>MLGTGPAAATTAATTSSNVSVLQQFASGLKSRNEETRAKAAKELQHYVTMELREMSQEESTRFYDQLNHHIFELVSSSDANERKGGILAIASLIGVEGGNATRIGRFANYLRNLLPSNDPVVMEMASKAIGRLAMAGDTFTAEYVEFEVKRALEWLGADRNEGRRHAAVLVLRELAISVPTFFFQQVQPFFDNIFVAVWDPKQAIREGAVAALRACLILTTQREPKEMQKPQWYRHTFEEAEKGFDETLAKEKGMNRDDRIHGALLILNELVRISSMEGERLREEMEEITQQQLVHDKYCKDLMGFGTKPRHITPFTSFQAVQPQQSNALVGLLGYSSHQGLMGFGTSPSPAKSTLVESRCCRDLMEEKFDQVCQWVLKCRNSKNSLIQMTILNLLPRLAAFRPSAFTDTQYLQDTMNHVLSCVKKEKERTAAFQALGLLSVAVRSEFKVYLPRVLDIIRAALPPKDFAHKRQKAMQVDATVFTCISMLARAMGPGIQQDIKELLEPMLAVGLSPALTAVLYDLSRQIPQLKKDIQDGLLKMLSLVLMHKPLRHPGMPKGLAHQLASPGLTTLPEASDVGSITLALRTLGSFEFEGHSLTQFVRHCADHFLNSEHKEIRMEAARTCSRLLTPSIHLISGHAHVVSQTAVQVVADVLSKLLVVGITDPDPDIRYCVLASLDERFDAHLAQAENLQALFVALNDQVFEIRELAICTVGRLSSMNPAFVMPFLRKMLIQILTELEHSGIGRIKEQSARMLGHLVSNAPRLIRPYMEPILKALILKLKDPDPDPNPGVINNVLATIGELAQVSGLEMRKWVDELFIIIMDMLQDSSLLAKRQVALWTLGQLVASTGYVVEPYRKYPTLLEVLLNFLKTEQNQGTRREAIRVLGLLGALDPYKHKVNIGMIDQSRDASAVSLSESKSSQDSSDYSTSEMLVNMGNLPLDEFYPAVSMVALMRIFRDQSLSHHHTMVVQAITFIFKSLGLKCVQFLPQVMPTFLNVIRVCDGAIREFLFQQLGMLVSFVKSHIRPYMDEIVTLMREFWVMNTSIQSTIILLIEQIVVALGGEFKLYLPQLIPHMLRVFMHDNSPGRIVSIKLLAAIQLFGANLDDYLHLLLPPIVKLFDAPEAPLPSRKAALETVDRLTESLDFTDYASRIIHPIVRTLDQSPELRSTAMDTLSSLVFQLGKKYQIFIPMVNKVLVRHRINHQRYDVLICRIVKGYTLADEEEDPLIYQHRMLRSGQGDALASGPVETGPMKKLHVSTINLQKAWGAARRVSKDDWLEWLRRLSLELLKDSSSPSLRSCWALAQAYNPMARDLFNAAFVSCWSELNEDQQDELIRSIELALTSQDIAEVTQTLLNLAEFMEHSDKGPLPLRDDNGIVLLGERAAKCRAYAKALHYKELEFQKGPTPAILESLISINNKLQQPEAAAGVLEYAMKHFGELEIQATWYEKLHEWEDALVAYDKKMDTNKDDPELMLGRMRCLEALGEWGQLHQQCCEKWTLVNDETQAKMARMAAAAAWGLGQWDSMEEYTCMIPRDTHDGAFYRAVLALHQDLFSLAQQCIDKARDLLDAELTAMAGESYSRAYGAMVSCHMLSELEEVIQYKLVPERREIIRQIWWERLQGCQRIVEDWQKILMVRSLVVSPHEDMRTWLKYASLCGKSGRLALAHKTLVLLLGVDPSRQLDHPLPTVHPQVTYAYMKNMWKSARKIDAFQHMQHFVQTMQQQAQHAIATEDQQHKQELHKLMARCFLKLGEWQLNLQGINESTIPKVLQYYSAATEHDRSWYKAWHAWAVMNFEAVLHYKHQNQARDEKKKLRHASGANITNATTAATTAATATTTASTEGSNSESEAESTENSPTPSPLQKKVTEDLSKTLLMYTVPAVQGFFRSISLSRGNNLQDTLRVLTLWFDYGHWPDVNEALVEGVKAIQIDTWLQVIPQLIARIDTPRPLVGRLIHQLLTDIGRYHPQALIYPLTVASKSTTTARHNAANKILKNMCEHSNTLVQQAMMVSEELIRVAILWHEMWHEGLEEASRLYFGERNVKGMFEVLEPLHAMMERGPQTLKETSFNQAYGRDLMEAQEWCRKYMKSGNVKDLTQAWDLYYHVFRRISKQLPQLTSLELQYVSPKLLMCRDLELAVPGTYDPNQPIIRIQSIAPSLQVITSKQRPRKLTLMGSNGHEFVFLLKGHEDLRQDERVMQLFGLVNTLLANDPTSLRKNLSIQRYAVIPLSTNSGLIGWVPHCDTLHALIRDYREKKKILLNIEHRIMLRMAPDYDHLTLMQKVEVFEHAVNNTAGDDLAKLLWLKSPSSEVWFDRRTNYTRSLAVMSMVGYILGLGDRHPSNLMLDRLSGKILHIDFGDCFEVAMTREKFPEKIPFRLTRMLTNAMEVTGLDGNYRITCHTVMEVLREHKDSVMAVLEAFVYDPLLNWRLMDTNTKGNKRSRTRTDSYSAGQSVEILDGVELGEPAHKKTGTTVPESIHSFIGDGLVKPEALNKKAIQIINRVRDKLTGRDFSHDDTLDVPTQVELLIKQATSHENLCQCYIGWCPFW[2x];>[2x]MNTSPGTVGSDPVILATAGYDHTVRFWQAHSGICTRTVQHQDSQVNALEVTPDRSMIAAAGYQHIRMYDLNSNNPNPIISYDGVNKNIASVGFHEDGRWMYTGGEDCTARIWDLRSRNLQCQRIFQVNAPINCVCLHPNQAELIVGDQSGAIHIWDLKTDHNEQLIPEPEVSITSAHIDPDASYMAAVNSTGNCYVWNLTGGIGDEVTQLIPKTKIPAHTRYALQCRFSPDSTLLATCSADQTCKIWRTSNFSLMTELSIKSGNPGESSRGWMWGCAFSGDSQYIVTASSDNLARLWCVETGEIKREYGGHQKAVVCLAFNDSVLG;>[2x]HHHHHHHHHHEQKLISEEDLDYKDDDDKMESEMLQSPLLGLGEEDEADLTDWNLPLAFMKKRHCEKIEGSKSLAQSWRMKDRMKTVSVALVLCLNVGVDPPDVVKTTPCARLECWIDPLSMGPQKALETIGANLQKQYENWQPRARYKQSLDPTVDEVKKLCTSLRRNAKEERVLFHYNGHGVPRPTVNGEVWVFNKNYTQYIPLSIYDLQTWMGSPSIFVYDCSNAGLIVKSFKQFALQREQELEVAAINPNHPLAQMPLPPSMKNCIQLAACEATELLPMIPDLPADLFTSCLTTPIKIALRWFCMQKCVSLVPGVTLDLIEKIPGRLNDRRTPLGELNWIFTAITDTIAWNVLPRDLFQKLFRQDLLVASLFRNFLLAERIMRSYNCTPVSSPRLPPTYMHAMWQAWDLAVDICLSQLPTIIEEGTAFRHSPFFAEQLTAFQVWLTMGVENRNPPEQLPIVLQVLLSQVHRLRALDLLGRFLDLGPWAVSLALSVGIFPYVLKLLQSSARELRPLLVFIWAKILAVDSSCQADLVKDNGHKYFLSVLADPYMPAEHRTMTAFILAVIVNSYHTGQEACLQGNLIAICLEQLNDPHPLLRQWVAICLGRIWQNFDSARWCGVRDSAHEKLYSLLSDPIPEVRCAAVFALGTFVGNSAERTDHSTTIDHNVAMMLAQLVSDGSPMVRKELVVALSHLVVQYESNFCTVALQFIEEEKNYALPSPATTEGGSLTPVRDSPCTPRLRSVSSYGNIRAVATARSLNKSLQNLSLTEESGGAVAFSPGNLSTSSSASSTLGSPENEEHILSFETIDKMRRASSYSSLNSLIGVSFNSVYTQIWRVLLHLAADPYPEVSDVAMKVLNSIAYKATVNARPQRVLDTSSLTQSAPASPTNKGVHIHQAGGSPPASSTSSSSLTNDVAKQPVSRDLPSGRPGTTGPAGAQYTPHSHQFPRTRKMFDKGPEQTADDADDAAGHKSFISATVQTGFCDWSARYFAQPVMKIPEEHDLESQIRKEREWRFLRNSRVRRQAQQVIQKGITRLDDQIFLNRNPGVPSVVKFHPFTPCIAVADKDSICFWDWEKGEKLDYFHNGNPRYTRVTAMEYLNGQDCSLLLTATDDGAIRVWKNFADLEKNPEMVTAWQGLSDMLPTTRGAGMVVDWEQETGLLMSSGDVRIVRIWDTDREMKVQDIPTGADSCVTSLSCDSHRSLIVAGLGDGSIRVYDRRMALSECRVMTYREHTAWVVKASLQKRPDGHIVSVSVNGDVRIFDPRMPESVNVLQIVKGLTALDIHPQADLIACGSVNQFTAIYNSSGELINNIKYYDGFMGQRVGAISCLAFHPHWPHLAVGSNDYYISVYSVEKRVR;>[2x]DEEERVFFMDDVE

pmcMechanistic target of rapamycin (mTOR, also known as mammalian TOR) is an essential serine/threonine protein kinase that responds to nutrients, growth factors, and cellular energy to promote cell growth. mTOR nucleates two distinct complexes, mTORC1 and mTORC2, each characterized by specific subunits, targets, downstream signaling pathways, and functions. mTORC1 contains mTOR, regulatory-associated protein of mTOR (RAPTOR), and mammalian lethal with SEC13 protein 8 (mLST8). RAPTOR binds mTORC1 substrates, including the well-characterized substrates ribosomal protein S6 kinase 1 (S6K1) and 4E binding protein 1 (4E-BP1), through a five-amino acid motif termed TOS. RAPTOR binds the LST2 TOS sequence to present LST2 to the kinase catalytic site in mTOR for phosphorylation of LST2 S670. mTORC1-dependent phosphorylation at S670 leads to monoubiquitination and stabilization of LST2.

To assess whether the LST2 TOS motif is functional, we examined whether a synthetic peptide corresponding to the LST2 TOS sequence binds RAPTOR. To further improve the resolution of the visualization of TOS motif interactions, we analyzed mTORC1 in complex with the synthetic LST2 TOS peptide, for which higher concentrations could be reached compared to full-length LST2. The LST2 TOS peptide contains three negatively charged residues which make electrostatic interactions with the positively charged TOS-binding pocket. F401 and M403 anchor the TOS peptide by binding in particularly deep cavities in the TOS-binding site, via hydrophobic interactions with surrounding residues. Finally, a comparison of LST2 TOS and previously described 4E-BP1 TOS binding shows that the TOS peptides, in particular, the consensus phenylalanine (F401 in LST2 and F114 in 4E-BP1), share a common mode of binding to the RAPTOR pocket. We performed fluorescence anisotropy with purified RAPTOR protein and a FITC-labeled LST2 TOS peptide including flanking residues (amino acids 395 to 407). The TOS peptide bound RAPTOR with a dissociation constant (Kd) of 330 nM. Thus, RAPTOR binds the LST2 TOS sequence with sub-micromolar affinity and LST2 F401 is critical for binding.> GSHMSYADSSRNAVLTNGGRTLRAECRNADGNWVTSELDLDTIIGNNDGHFQWGGQ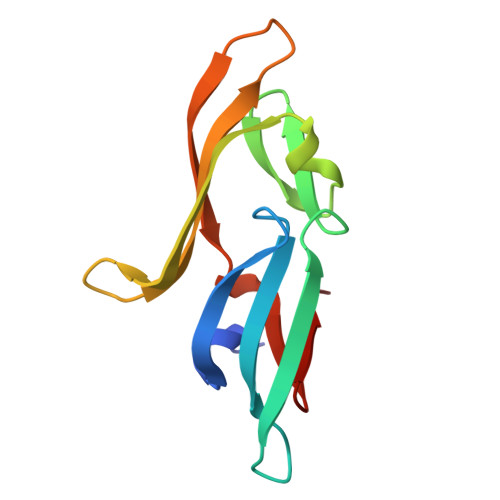NFTETAEDIRFHPKEGAAEQPILRARLRDCNGEFHDRDVNLNRIQNVNGRLVFQ> MANRTVKDAHSIHGTNPQYLVEKIIRTRIYESKYWKEECFGLTAELVVDKAMELRFVGGVYGGNIKPTPFLCLTLKMLQIQPEKDIIVEFIKNEDFKYVRMLGALY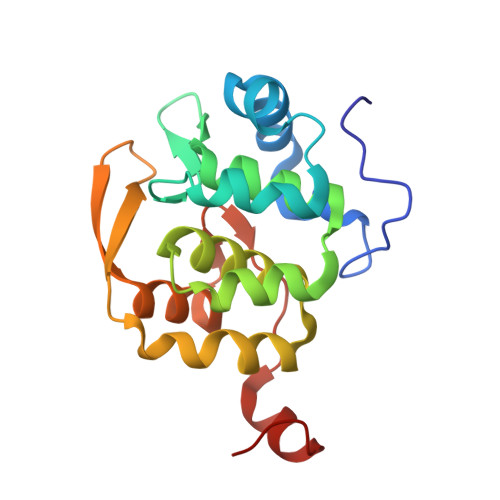MRLTGTAIDCYKYLEPLYNDYRKIKSQNRNGEFELMHVDEFIDELLHSERVCDIILPRLQKRYVLEEAEQLEP> FHLTTRGGEPHMIVSKQERGKSLLFKTSAGVNMCTLIAMDLGELCEDTMTYKCPRITETEPDDVDCWCNATETWVTYGTCSQTGEHRRDK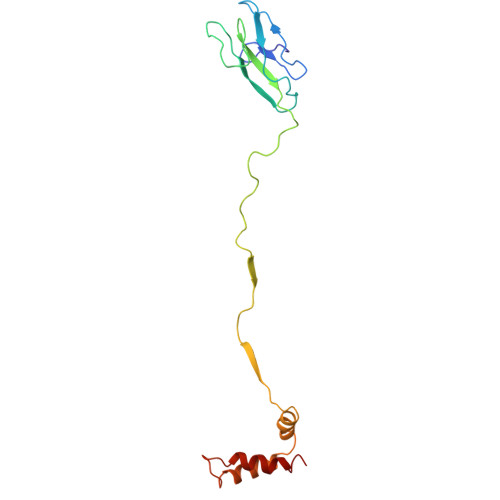RSVALAPHVGLGLETRTETWMSSEGAWKQIQKVETWALGHPGFTVIALFLAHAIGTSITQKGIIFILLMLVTPSMA>[2x]GSSMVTGGMASKWDQKGMDIAYEEALLGYKEGGVPIGGCLINNKDGSVLGRGHNMRFQKGSATLHGEISTL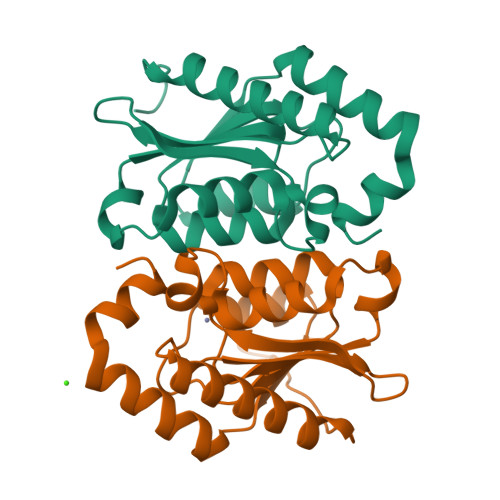ENCGRLEGKVYKDTTLYTTLSPCDMCTGAIIMYGIPRCVVGENVNFKSKGEKYLQTRGHEVVVVDDERCKKLMKQFIDERPQDWFEDIGE> LKIAAFNIQTFGETKMSNATLVSYIVQILSRYDIALVQEVRDSHLTAVGKLLDNLNQDAPDTYHYVVSEPLGRNSYKERYLFVYRPDQVSAVDSYYYDDGCEPCGNDTFNREPAIVRFFSRFTEVREFAIVPLHAAPGDAVAEIDALYDVYLDVQEKWGLEDVMLMGDFNAGCSYVRPSQWSSIRLWTSPTFQWLIPDSADTTATPTHCAYDRIVVAGMLLRGAVVPDSALPFNFQAA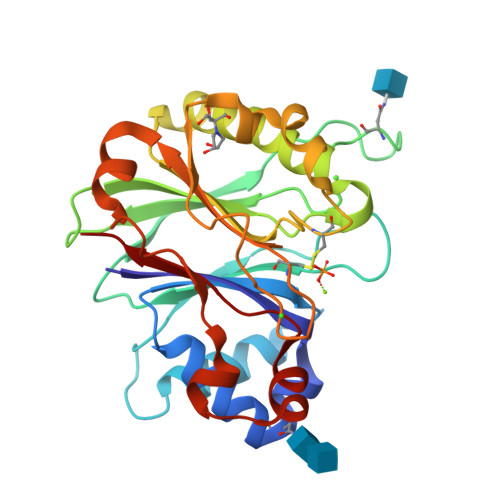YGLSDQLAQAISDHYPVEVMLK>GSEPCVEVVPNITYQCMELNFYKIPDNLPFSTKNLDLSWNPLRHLGSYSFFSFPELQVLDLSRCEIQTIEDGAYQSLSHLSTLILTGNPIQSLALGAFSGLSSLQKLVAVETNLASLENFPIGHLKTLKELNVAHNLIQSFKLPEYFSNLTNLEHLDLSSNKIQSIYCTDLRVLHQMPLLNLSLDLSLNPMNFIQPGAFKEIRLKELALDTNQLKSVPDGIFDRLTSLQKIWLHTNPWDCSCPRIDYLSRWLNKNSQKEQGSAKCSGSGKPVRSIICPT[2x];>[2x]GSQKQYWVCNSSDASISYTYCDKMQYPISINVNPCIELKGSKGLLHIFYIPRRDLKQLYFNLYITVNTMNLPKRKEVICRGSDDDYSFCRALKGETVNTTISFSFKGIKFSKGKYKCVVEAISGSPEEMLFCLEFVILHQPN

Toll-like receptor 4 (TLR4), a superfamily of LRR proteins, is the principal receptor mediating innate immune responses against infections by Gram-negative bacteria. In this process, myeloid differentiation protein 2 (MD2) recognizes various lipopolysaccharides (LPSs) released from the Gram-negative bacteria, forming a complex with LPS at its hydrophobic pocket. In an attempt to prevent the systemic immune response caused by LPS, a TLR4 decoy receptor was constructed by combining LRR modules from the TLR4 ectodomain and VLR. The constructed decoy receptor was shown to attenuate the TLR4-mediated signaling process by trapping MD2, implicating a potential therapeutics for bacteria-induced sepsis and inflammation.

Phe-63 was substituted for tryptophan and leucine for the interaction with Ile-66 in MD2. To get detailed information on interacting interfaces, we attempted to determine the crystal structures of three single variants (M41E, F63W, V134L) in complex with MD2 in the presence of Eritoran. It was shown that Eritoran, derived from the lipid A structure of Rhodobacter sphaeroides LPS, is critical for crystallizing the decoy receptor/MD2 complex. We obtained the crystals of three mutants in complex with MD2 and Eritoran. The F63W mutant /MD2 complex structure was determined at a 3.6 Å resolution and the others at lower resolution. Even at this moderately low resolution, the density maps clearly reveal backbone structure and some side chains. Especially, we could determine the side chain position of the mutated F63W residue and interaction with Arg-68 of MD2. The complex structure of the F63W mutant displayed that Trp-63 was closely positioned to form a cation-π interaction with Arg-68 on MD2, confirming our design strategy. The crystal structures of three single mutants revealed that mutated residues have interactions with the target protein (MD2) as we designed, which confirms that our design strategy works well.> AAVINTFDGVADYLQTYHKLPDNYITKSEAQALGWVASKGNLADVAP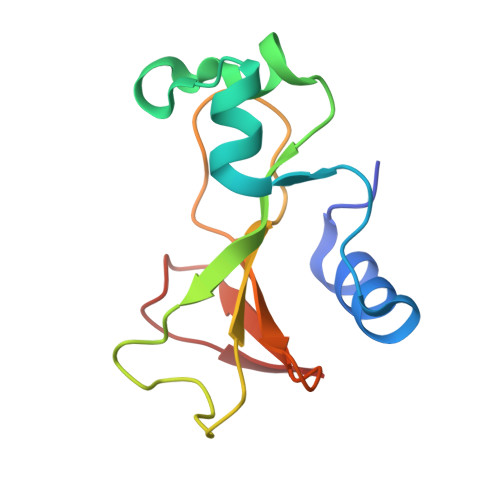GKSIGGDIFSNREGKLPGKSGRTWREADINYTSGFRNSDRILYSSDWLIYKTTDHYQTFTKIR> MSSALTDLFPLPIVQAPMAGGVSVPQLAAAVCEAGGLGFLAAGYKTADGMYQEIKRLRGLTGRPFGVNVFMPQPELAESGAVEVYAHQLAGEAAWYETELGDPDGGRDDGYDAKLAVLLDDPVPVVSFHFGVPDREVIARLRRAGTLTLVTATTPEEARAVEAAGADAVIAQGVEAGGDQGTHRDSSEDDGAGIGLLSLLAQVREAVDIPVVAAGGIMRGGQIAAVLAAGADAAQLGTAFLATDESGAPGPHKRALTDPLFARTRLTRAFTGRPARSLVNRFLREHGPYAPAAYPDVHHLTSPLRKAAAKAGDAQGMALWAGQGHRMARELPAGRLVEVLAAELAEARTALSDASRENES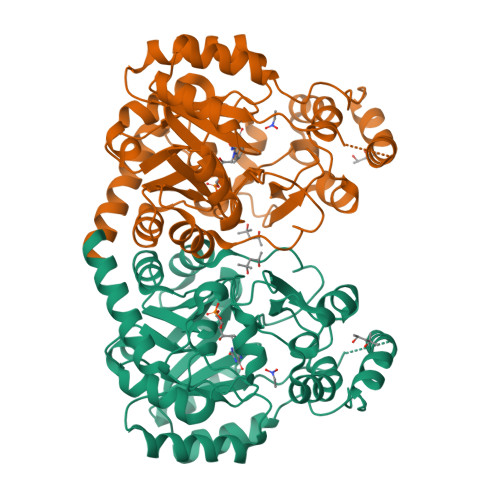RKGHHHHHH> NEEGFFFSARGHRP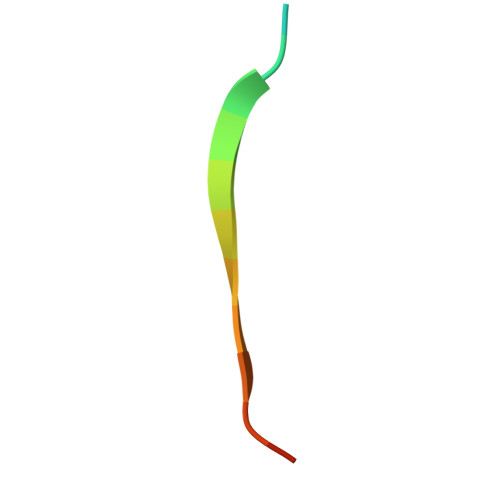LD Here we present four in situ and one isolated cryoEM structures of the trimeric spike of the cytoplasmic polyhedrosis virus, a member of the non-enveloped Reoviridae family and a virus historically used as a model in the discoveries of RNA transcription and capping. CPV has two functionally essential components located along the icosahedral 5-fold axis: the RNA-dependent RNA polymerase (RdRp) inside and the RNA capping turret outside;25,27 a trimeric spike is attached to the latter. Each spike monomer has four domains: N-terminal, body, claw, and C-terminal.

In the closed spike, the tip of the claw domain that contains the membrane fusion loops points toward the capsid direction, with the RGD-containing CTD visible, though covered; in the opened spike, the claw domain rotates ~96° and points away from the capsid, while the CTD becomes likely flexible, as it becomes invisible in our structure. The root of the trimeric spike plugs into the iris of the pentameric turret like a bottle cork. The final part of the monomer, the CTD, is a helix-turn-helix. Within the trimeric spike of CPV, it is sandwiched by the body sub-domain 2 of the same subunit and the claw domain of the adjacent subunit through complementary surface charge. However, the RGD motif of the CPV trimeric spike is covered in the putative penetration-inactive state (i.e., closed spike) and exposed in the putative penetration-active state (i.e., opened spike), while the integrin-binding motifs known in other viruses are always exposed. In our structures of the CPV trimeric spike, we observed the PPPDE core in the body sub-domain 2, though its active site is buried inside the trimeric spike. Additionally, we extracted free spikes already detached from the virions, visible in the background of the SA-CPV micrographs. The reconstruction result shows that the majority of these particles are in closed spike conformation, indicating that the conformational change of the trimeric spike was not caused by spike detachment from the virion.

> MEINRAEIRREITRYTGLIEQQTQLNISDNDENILKTLIADYNLRMRRDALLGELARLDELRDISQVKGVEYKVTIPLLPVISTLNQHEFEITQANIETDFIADNVTFVTSFVPADLDLEQTIQRVFFRTTATTPHFQSFNLVIEILNYDQDSGDVELHVKIMIVRPNSDVVNYDYTWIGKDYERISVCYNLISHLQRIDGPHGRDDEAEMPIYRIIRRDSGSIPSYASGEHLYVISSHLHVDEIVRRREHKSISVDVTQLSLILPIIRTFNPVDLREVRIEDITPGIEFTINMEVSTYLAESSGSHVDMQRAIMNHADKIVGNYTGQQWNVQSNMLSEVRTQMLEEEDEEARQRGDYTTSTLVQTMAQVSDLFSSTILYRRAEARLDNTVGAFELLRPVLSIPSEYVHNGRVGPITNIPANASIVTSSSSGAGQVRNIFKPIGDQTINESHFANVFSNDEYAIYLRFSYRQAPVQSETVYLQQNLPSMRIVSPSSVSTTVSTAVIGGNTIHINCPIRPHREDRLVSGGVQVPRQSTAVEIRVQEILIGYRQATTFPIDTEGRLSLELMYGLESRSAVGNTMSPVRFVTVNDGEFFGLTCPIDLTLSTVVDPSSYLSDGVILVATAFEDLRGYAWVATLGGDWPRTYNSSMRAFNVLTGGDINLSTEYGSEMTYTFKVELPIVYMFNNMTVISNNVPRVPVLGVTYASIYQDSRTELEARRFLQTLVFRIHGNWSARIPYTPGNLPTRNTANQHQDIQQVINDSISQELGRLSDELLNMKNRLDHLERQFEMFIQSQESEWWEILLNVVMDTVLGYFSTFAGNALKSAQQAISKAVGYTRRVLMTVTKTMRNGPIFTRLLGAKNLSGQALASLETLVESVLRSINVKKSRFMSGAEPLYKNNKVAQHIDNTEKMNMMMDFSFANRNNRQNITADTLSRMHTQNAHGTSDTVLPAMRVYYRPLGFLDKRVGEALHKGITRPEALKKQLRSDVANVGTRAPSHAFMTYTDVLYEDAGSYIVSKRYLGIGELNRFGRTTSDKNADIGGVNIKYRVNKITADGKYIIDRLSHTESGYTAADVDRLYRSLFGKQGDGLSTEQKWMDISRGVDAKIISADMVSEEFLSSKYTGQMIDELINSPPQFNYSLIYRNCQDFVLDVLRVAQGFSPSNKWDVSTAARMQQRRVISLMDDLMSESETFARSAHSNHSLLQQIRRSYVKARKRGDLHTVKALQLRLKGFFQI> VGGQQRYNVKPRQPEYKCIDSNLQYDCVFYDVHIDMQTQDVYFGFEDITLNNQKIVTFKNSTMRKLPAALLDSFRQVELLNLNDLQIEEIDTYAFAYAHTIQKLYMGFNAIRYLPPHVFQNVPLLTVLVLERNDLSSLPRGIFHNTPKLTTLSMSNNNLERIEDDTFQATTSLQNLQLSSNRLTHVDLSLIPSLFHANVSYNLLSTLAIPIAVEELDASHNSINVVRGPVNVELTILKLQHNNLTDTAWLLNYPGLVEVDLSYNELEKIMYHPFVKMQRLER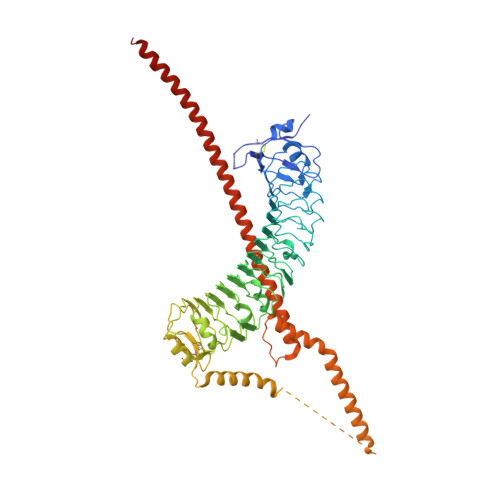LYISNNRLVALNLYGQPIPTLKVLDLSHNHLLHVERNQPQFDRLENLYLDHNSIVTLKLSTHHTLKNLTLSHNDWDCNSLRALFRNVARPAVDDADQHCKIDYQLEHGLCCKESDKPYLDRLLQYIALTSVVEKVQRAQGRCSATDTINSVQSLSHYITQQGGVPLQGNEQLEAEVNELRAEVQQLTNEQIQQEQLLQGLHAEIDTNLRRYRLPKDGLARSSDNLNKVFTHLKERQAFKLRETQARRTEADAKQKETEDLEQENIALEKQLDNKRAKQAELRQETSLKRQKVKQLEAKKNRNPDTRRVSHHHHHH IMP-13, a member of subgroup 2, sharing 92.3% amino acid sequence similarity with IMP-2 and 82.5% with IMP-1 (Fig. SI2), was first identified in the Gram-negative pathogen Pseudomonas aeruginosa from clinical samples in Italy and is a common cause of carbapenem resistance, often involved in large outbreaks. Imipenemases represent one of the major groups of class B1 metallo-β-lactamases found in Gram-negative pathogens, and these enzymes can hydrolyze all bicyclic β-lactam antibiotics. The overall protein architecture of the IMP-13 apo structure is consistent with that of the previously published metallo-β-lactamase fold, consisting of a global αβ/βα topology with a shallow active-site cleft at the border of the two β-sheets. The structural information and dynamics presented here reveal important information about the mechanism of antibiotic binding, as well as a significant role for the active-site-covering loop (L1), indicating that the plasticity of the active-site region is important for the broad substrate recognition spectrum of these enzymes.

The most solvent-exposed parts of the four antibiotics are very distinct, while in addition, imipenem has no pyrrolidine ring in the antibiotic tail. The terminal part of the imipenem tail was modeled in three different conformations (50%:25%:25% occupancy), highlighting the extreme flexibility of this moiety. Due to the different conformers, the interaction network is different in every modeled position: conformer A creates a hydrogen bond with the backbone carbonyl of Val30 and water-mediated hydrogen bonds with the backbone of Thr32. The most solvent-exposed conformation, conformer B, lacks interactions with surrounding residues, most likely interacting with a water network, while conformer C interacts with the wider water network. In addition, Trp28 shows interactions with the pyrroline methyl group (C-21), present in all the antibiotics studied other than imipenem. The lack of this interaction in imipenem could lead to a reduction in binding interactions to the loop and may contribute to the observed reduction in affinity (increase in Km) for imipenem. In contrast, imipenem lacks this additional methyl group, which reduces the strength of the lipophilic interaction with the Trp28 side chain, thus resulting in greater loop flexibility. Furthermore, as shown by both shorter and longer overall simulation times for all the complexes, the tail of imipenem shows high flexibility and occupies multiple rotamer positions; thus, it does not contribute further to the loop stability. In contrast, imipenem shows weaker binding (Km, ca. 50 μM), consistent with the higher L1 flexibility. Notably, the kcat for imipenem is 2 orders of magnitude higher than that for meropenem and ertapenem.

>[2x]GALPDLKIEKLEEGVFVHTSFEEVNGWGVVTKHGLVVLVNTDAYLIDTPFTATDTEKLVNWFVERGYEIKGTISSHFHSDSTGGIEWLNSQSIPTYASELTNELLKKSGKVQAKYSFSEVSYWLVKNKIEVFYPGPGHTQDNLVVWLPESKILFGGCFIKPHGLGNLGDANLEAWPKSAKILMSKYGKAKLVVSSHSEKGDASLMKRTWEQALKGLKESKKTSSPSN>TAPSQVLKIRRPDDWHLHLRDGDMLKTVVPYTSEIYGRAIVMPNLAPPVTTVEAAVAYRQRILDAVPAGHDFTPLMTCYLTDSLDPNELERGFNEGVFTAAKLYPANATTNSSHGVTSVDAIMPVLERMEKIGMPLLVHGEVTHADIDIFDREARFIESVMEPLRQRLTALKVVFEHITTKDAADYVRDGNERLAATITPQHLMFNRNHMLVGGVRPHLYCLPILKRNIHQQALRELVASGFNRVFLGTDSAPHARHRKESSCGCAGCFNAPTALGSYATVFEEMNALQHFEAF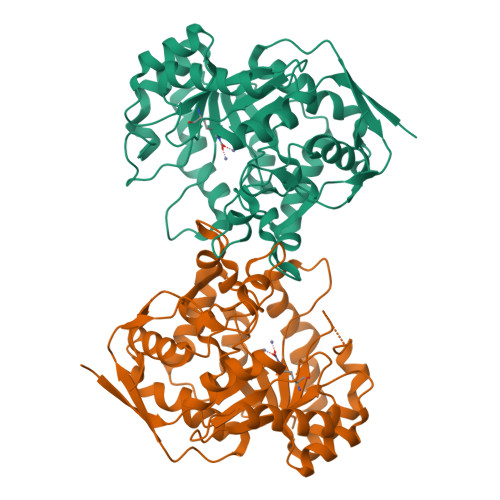CSVNGPQFYGLPVNDTFIELVREEQQVAESIALTDDTLVPFLAGETVRWSVKQ[2x]(2R)-2-{[(S)-[(1R)-1-amino-2-phenylethyl](hydroxy)phosphoryl]methyl}butanedioic acid | C13 H18 N O6 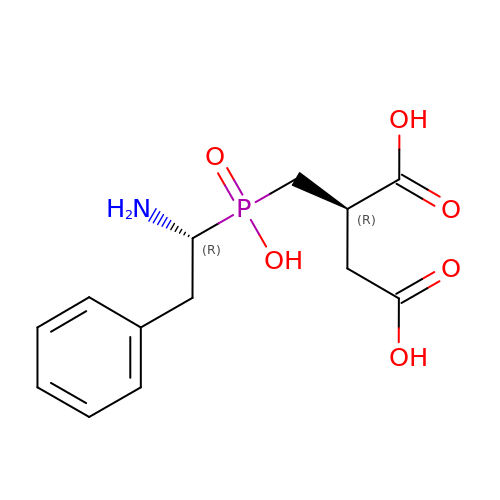P | HUMGCALEJILOSC-WDEREUQCSA-N>SGTVTFDITNISHKAIDIILKVVLGIAEHEGTEVTFHSERGQLQIEVKNLHEEDKRLIEQAIEAARLADSPDPESVARAVELLTKVAKASTNTELIQFIVKELLELARKLTDPKDLAKVLDSISELLTELALKTGDPTAALAAMVAHIAELVVRLALMAERTHPGSEIVKKAVKLVQEVAEEVLEAAQLMLEKPNSDEVAKKLEEVAKKAIEACIELQQILEAWAKERGDQDLLREVREHKLQILTIAVAYKAAQMGVTVLKHTHGWVV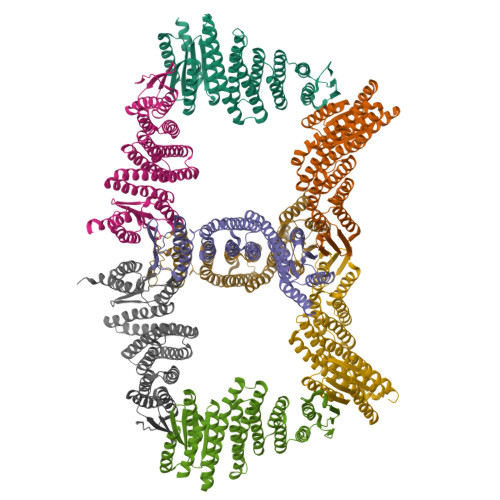FLVILGLHKQQAEQLLRFVHRVAHALGVTLSITFSGDIVVIAVTVGASEEEKKEVRKIVKEIAKQLRHAETEEEAKEIVQRVIEEWQEEGGSG[8x]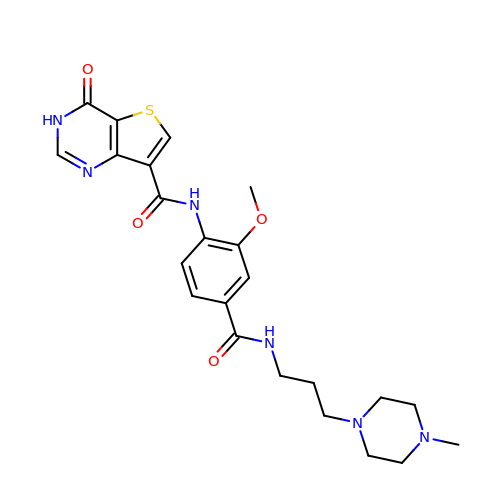N-(2-methoxy-4-{[3-(4-methylpiperazin-1-yl)propyl]carbamoyl}phenyl)-4-oxo-3,4-dihydrothieno[3,2-d]pyrimidine-7-carboxamide | C23 H28 N6 O4 S | YTKZLQGZFHCSKQ-UHFFFAOYSA-N>[2x]VHHPPSYVAHLASDFGVRVFQQVAQASKDRN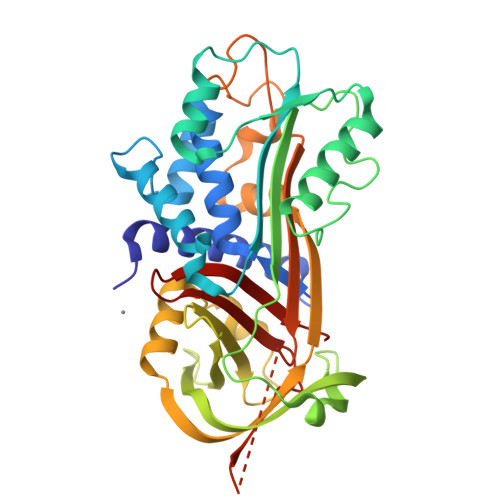VVFSPYGVASVLAMLQLTTGGETQQQIQAAMGFKIDDKGMAPALRHLYKELMGPWNKDEISTTDAIFVQRDLKLVQGFMPHFFRLFRSTVKQVDFSEVERARFIINDWVKTHTKGMISNLLGKGAVDQLTRLVLVNALYFNGQFKTPFPDSSTHRRLFHKSDGSTVSVPMMAQTNKFNYTEFTTPDGHYYDILELPYHGDTLSMFIAAPYEKEVPLSALTNILSAQLISHWKGNMTRLPRLLVLPKFSLETEVDLRKPLENLGMTDMFRQFQADFTSLSDQEPLHVAQALQKVKIEVNESGTVASSSTAVIVSARMAPEEIIMDRPFLFVVRHNPTGTVLFMGQVMEP>GSHMSETDLLMKMVRQPVKLYSVATLFHEFSEVITKLEHSVQKEPTSLLSEENWHKQFLKFAQALPAHGSASWLNLDDALQAVVGNSRSAFLHQLIAKLKSRHLQVLELNKIGSEPLDLSNLPAPFYVLLPESFAARITLLVQDKALPYVRVSME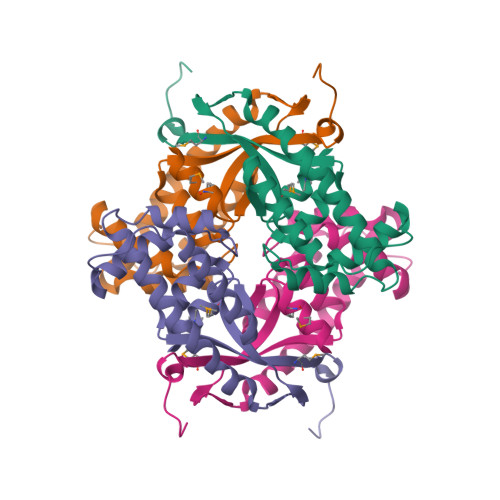YWHALEYKGELNDPAANKARKEAELAAATAEQ[2x]>GSHMESFLLSKVSFVIKKIRLEKGMTQEDLAYKSNLDRTYISGIERNSANLTIKSLELIMKGLEVSDVVFFEMLIKEILKHD[2x]

The most widespread of these mechanisms employs a “controller” (C) protein encoded by a gene downstream of its own promoter, and usually co-transcribed with the endonuclease (R) gene as a single transcriptional unit. The C-protein binds at various sites within the C/R promoter to regulate transcription of its own gene and the associated endonuclease gene. Unusually, in the RM system Esp1396I, the C-protein also represses the MTase (M) gene by binding to the promoter at the transcriptional start site, denoted OM where the C/R genes and the M gene are transcribed convergently from different promoters. Flexibility in this loop is very important for DNA sequence recognition, as it has been observed in the nucleoprotein structures to adopt different conformations depending on which operator site the protein is bound to.

The mutant proteins Y37F, Y37A, T36A, S52A and R46A were crystallized (the latter in two different space groups) and the crystals diffracted X-rays to a resolution of 1.5–2.0 Å. The KD for the R46A mutant was ∼30 fold greater than that of the wild type, showing a much weaker interaction with the OM operator site, and consistent with a key DNA-binding role for this arginine side chain. The ΔΔG for R46A is significantly larger (8.5 kJ mol−1), and that for the T36A mutation must be larger still, since we could not measure any DNA binding activity of this mutant protein. Both R46 and T36 of C.Esp1396I are seen in crystal structures of DNA-protein complexes to interact directly with the base pairs involved in sequence recognition, specifically with the G and C bases, respectively, of the C-box recognition sequence GTC. Five of the monomers in the asymmetric unit are observed to be in loop conformation I but the sixth more closely resembles that of conformation II, which is almost identical to that in the DNA-protein complex with the 19OM operator site. Both of the R46A crystal structures and the S52A crystal structure have adopted loop conformation III, despite the varying buffer conditions and crystallographic interactions in those three structures. The SO4 based interaction observed in the high-resolution wild type structure is also observed in the Y37A, S52A and monoclinic R46A structures. Both the monoclinic R46A and S52A structures show almost identical crystal contacts to those of the triclinic wild type protein, even though the space group and unit cell are different. The CC1/2 value was not determined for the monoclinic R46A structure.> MSNVYVMALDFGNGFVKGKINDEKFVIPSRIGRKTNENNQLKGFVDNKLDVSEFIINGNNDEVLLFGNDLDKTTNTGK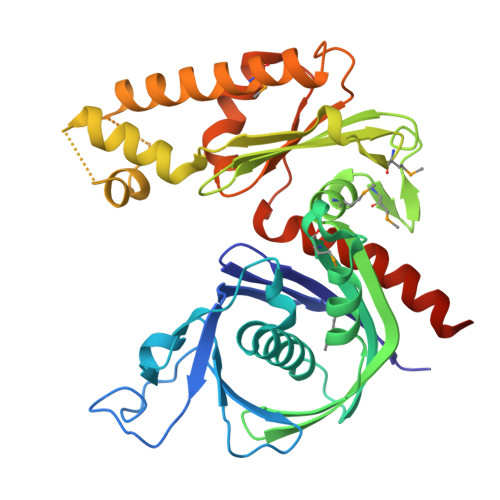DTASTNDRYDIKSFKDLVECSIGLLAREVPEEVVNVVIATGMPSNEIGTDKQAKFEKLLNKSRLIEIDGIAKTINVKGVKIVAQPMGTLLDLNMENGKVFKAFTEGKYSVLDFGSGTTIIDTYQNMKRVEEESFVINKGTIDFYKRIASHVSKKSEGASITPRMIEKGLEYKQCKLNQKTVIDFKDEFYKEQDSLIEEVMSNFEITVGNINSIDRIIVTGGGANIHFDSLSHYYSDVFEKADDSQFSNVRGYEKLGELLKNKVEQESKRGSHHHHHH> TENIISVDHLTYQYDENQAPALTDVSFTVHAGEWLAIVGH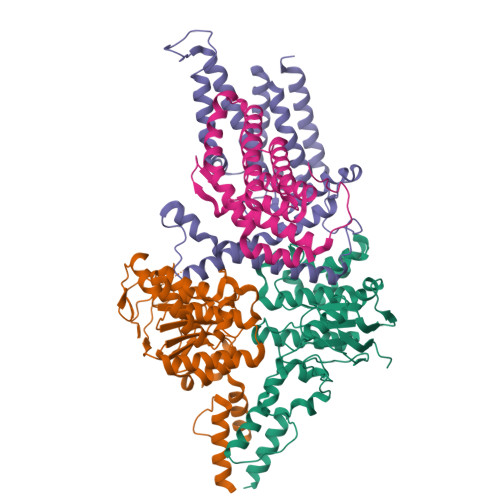NGSGKSTLAKSLDGLLPFTQGSVTVGGITLTPETVWQVREQIGMIFQNPDNQFVGATVEDDVAFGLENRQISRDEMVPRVQAALAQVGMTSFAQREPSSLSGGQKQRVALAGIVAIAPKILILDEATSMLDPQGRIEMLAIVRQLRQQQNLTVISITHDIDEAASADRVLVIDDGRLVDEAVPSQIFERGTQLVEMGLDLPFTEKLKAALRQRGITPPTTYQTAAEMEEWLWQSLSNT;> AIAFEHVTYTYQAGTPMAHTALTDVSLTVPDRGYLAIIGHTGSGKSTLIQQLNALLKPTSGTIKIDEFTITPETTNAALKPLRQHVGMVFQFPENQLFEETVRQDIAFGPKNFGMADADALALADEMLTTVGLDQSYAERSPFELSGGQMRRVAIAGVLAMQPKVLVLDEPTAGLDPQGRQEMMRLFARLHQEQGLTIVLVTHQMEDVAQYAEQVAVMHEGRLMKFGTPADVFSNREWLQDHQLDVPQAAQFARRLRDRGLTFPKQPLTADQLADYLAQQWAQRGADHV;> MSNFIFGRYLPLDSVVHRLDPRAKLMLSFCYIIVVFLANNIWSYAILIAFTVGAILSSKISLGFFLKGIRPLLWLIVFTVVLQLLFSPAGGHTYFHWAFINVTQDGLINAGYIFVRFLLIIMMSTLLTLSTQPLDIATGLASLMKPLRWVKVPVDTLAMMLSIALRFVPTLMDEATKIMNAQRARGVDFGEGGLFKQAKSLIPLMVPLFMSAFNRAEDLSTAMEARGYQDSEHRSQYRILTWQRRDTVTWLLFLLGFVAILIFRHW;> MKTMAKTQLPKLDTLSMVTMGVLMALQLVISRFSVGNNFIKVSFTFLIVALIAKWFGPWWGMLTAAVVDVIGTLMTGGPFFIGFTVSAVLGSLIYAVFLYRQPVSWWRVIGASVLIALLVNTLLNTLWVTIMYQTPFWSLLPVRALKELIVTPVQIVLVYLLLKSQVIQMIQARLNK> EPIRLPNPMIGFGVPNEPGLITHRSLPELARGPPFFYYENVALTPKGVWETISRHLFEIPPEFVDSKYFCVAARKRGYIHNLPINNRFQIQPPPKYTIHDAFPLSKRWWPEWDKRTKLNCILTCTGSAQLTNRIRVALEPYNEEPEPPKHVQRYVIDQCKKWNLVWVGKNKAAPLEPDEMESILGFPKNHTRGGGMSRTERFKSLGNSFQVDTVAYHLSVLKPIFPHGINVLSLFTGIGGGEVALHRLQIKMKLVVSVEISKVNRNILKDFWEQTNQTGELIEFSDIQHLTNDTIEGLMEKYGGFDLVIGGSPCNNLAGGNRVSRVGLEGDQSSLFFEYCRILEVVRARMRGS

Here, we report structural and biochemical characterizations of the intrinsic substrate preference of DOMAINS REARRANGED METHYLTRANSFERASE 2 (DRM2), a plant DNA methyltransferase responsible for establishing all cytosine methylation and maintaining CHH methylation. In plants, the establishment of DNA methylation in all sequence contexts is mediated by DOMAINS REARRANGED METHYLTRANSFERASE 2 (DRM2), following an RNA-directed DNA methylation pathway. As previously observed, The DRM2 MTase domain is composed of a catalytic core adopting a Rossmann fold and a loop-rich target recognition domain (TRD), creating a catalytic cleft to embed the DNA duplex. Among nine CHH motifs, the DRM2 methyltransferase (MTase) domain shows marked substrate preference toward CWW (W = A or T) motifs, correlating well with their relative abundance in planta.

To address this, we solved the crystal structure of the DRM2 MTase domain in complex with a DNA duplex mimicking the CTA DNA used for the in vitro DNA methylation assay, except that the target cytosine was replaced by a 5-fluorocytosine (fC) to ensure the formation of a stable, covalent complex between DRM2 and DNA. The crystal structure of the DRM2-CTA complex bound to cofactor by-product S-adenosyl-homocysteine (SAH) was refined to 2.91 Å resolution, with each asymmetric unit containing one complex. Consistent with what was observed for other DRM2-DNA complexes, the catalytic loop (residues 585–596) of DRM2 enters the DNA minor groove, with residue R595 intercalating into the A11′pG10′ step on the non-target strand; on the other hand, a loop–helix (αA)–helix (αB) (LHH) motif of the TRD occupies the DNA major groove centered around the (fC)TA motif. As a result, the major conformation (conformation I, relative population of ∼0.55) manifests greater inter-strand distances for the T12′pA11′ step than the minor conformation (conformation II, relative population of ∼0.45). Detailed comparison of the two alternative conformations of the DRM2-bound CTA DNA reveals that Thy12′ undergoes a negative propeller twist from conformation II to conformation I (36.5° vs 29.6°), resulting in a greater inter-base pair stacking for the T12′pA11′ step (136 Å2 in conformation I vs 121 Å2 in conformation II). Such a difference in base-stacking interaction between the two conformational states is accompanied by a differential interaction between the CTA DNA and the TRD of DRM2: In conformation II, Thy12′ and Ade11′ are in proximity with the TRD, reminiscent of what was observed for the DRM2-CTT complex. In contrast, the corresponding region in the conformation I moves away from TRD by ∼4 Å, resulting in an increase of the distance between S400/R406 and the backbone of Thy12′ to 6.2 Å and 7.5 Å, respectively, in the conformation I.>GPLGSMGKKSRVKTQKSGTGATATVSPKEILNLTSELLQKCSSPAPGPGKEWEEYVQIRTLVEKIRKKQKGLSVTFDGKREDYFPDLMKWASENGASVEGFEMVNFKEEGFGLRATRDIKAEELFLWVPRKLLMTVESAKNSVLGPLYSQDRILQAMGNIALAFHLLCERASPNSFWQPYIQTLPSEYDTPLYFEEDEVRYLQSTQAIHDVFSQYKNTARQYAYFYKVIQTHPHANKLPLKDSFTYEDYRWAVSSVMTRQNQIPTEDGSRVTLALIPLWDMCNHTNGLITTGYNLEDDRCECVALQDFRAGEQIYIFYGTRSNAEFVIHSGFFFDNNSHDRVKIKLGVSKSDRLYAMKAEVLARAGIPTSSVFALHFTEPPISAQLLAFLRVFCMTEEELKEHLLGDSAIDRIFTLGNSEFPVSWDNEVKLWTFLEDRASLLLKTYKTTIEEDKSVLKNHDLSVRAKMAIKLRLGEKEILEKAVKSAAVNREYYRQQMEEKAPLPKYEESNLGLLESSVGDSRLPLVLRNLEEEAGVQDALNIREAISKAKATENGLVNGENSIPNGTRSENESLNQESKRAVEDAKGSSSDSTAGVKE[2x];>TLKYPIEHGI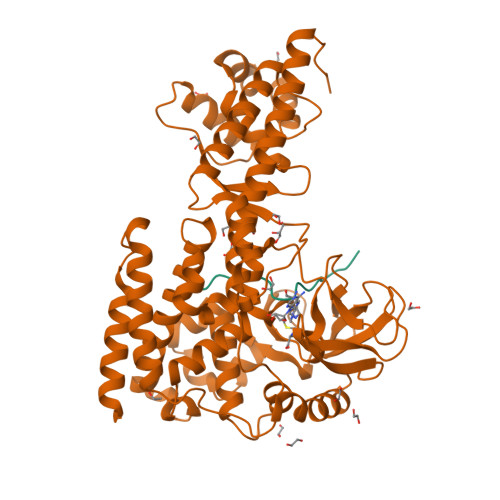VTNWD[2x]> ACEM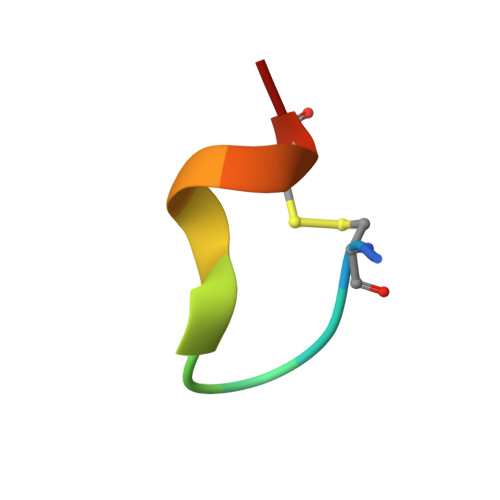GFFQDCGX>SMNFYSAYQHGFVRVAACTHHTTIGDPAANAASVLDMARACHDDGAALAVFPELTLSGYSIEDVLLQDSLLDAVEDALLDLVTESADLLPVLVVGAPLRHRHRIYNTAVVIHRGAVLGVVPKSYLPTYREFYERRQMAPGDGERGTIRIGGADVAFGTDLLFAASDLPGFVLHVEICEDMFVPMPPSAEAALAGATVLANLSGSPITIGRAEDRRLLARSASARCLAAYVYAAAGEGESTTDLAWDGQTMIWENGALLAESERFPKGVRRSVADVDTELLRSERLRMGTFDDNRRHHRELTESFRRIDFALDPPAGDIGLLREVERFPFVPADPQRLQQDCYEAYNIQVSGLEQRLRALDYPKVVIGVSGGLDSTHALIVATHAMDREGRPRSDILAFALPGFATGEHTKNNAIKLARALGVTFSEIDIGDTARLMLHTIGHPYSVGEKVYDVTFENVQAGLRTDYLFRIANQRGGIVLGTGDLSELALGWSTYGVGDQMSHYNVNAGVPKTLIQHLIRWVISAGEFGEKVGEVLQSVLDTEITPELIPTGEEELQSSEAKVGPFALQDFSLFQVLRYGFRPSKIAFLAWHAWN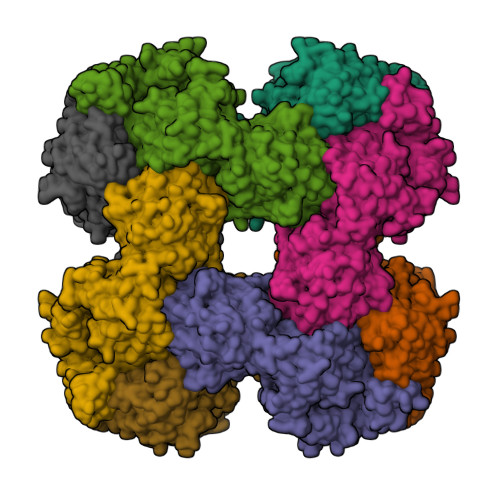DAERGNWPPGFPKSERPSYSLAEIRHWLQIFVQRFYSFSQFKRSALPNGPKVSHGGALSPRGDWRAPSDMSARIWLDQIDREVPKG[4x]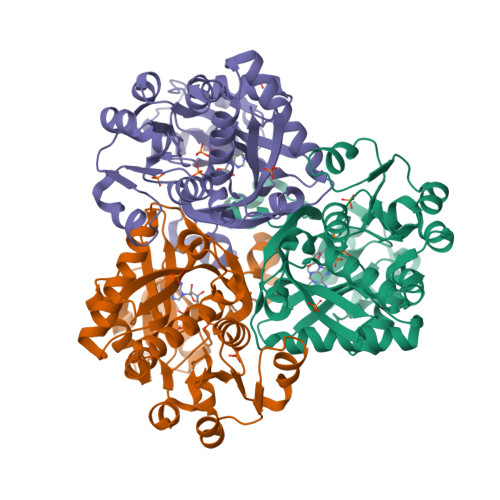>[6x]MKVRIATYASHSALQILKGAKDEGFETIAFGSSKVKPLYTKYFPVADYFIEEKYPEEELLNLNAVVVPTGSFVAHLGIELVENMKVPYFGNKRVLRWESDRNLERKWLKKAGIRVPEVYEDPDDIEKPVIVKPHGAKGGKGYFLAKDPEDFWRKAEKFLGIKRKEDLKNIQIQEYVLGVPVYPHYFYSKVREELELMSIDRRYESNVDAIGRIPAKDQLEFDMDITYTVIGNIPIVLRESLLMDVIEAGERVVKAAEELMGGLWGPFCLEGVFTPDLEFVVFEISARIVAGTNIFVNGSPYTWLRYDRPVSTGRRIAMEIREAIENDMLEKVLT> MQNWTLVWQDEFTNGISSDWVFETGNGNSGWGNNELQYYRRENATVENGNLVITAKRESIGGYNYTSTRMKTQGRKSWKYGKVEARIAMPSFMGSWPAFWMLGDNISSVGWPACGAIDIMEHVNTEAQTHGTIHWQDHNNTYANYSGSIP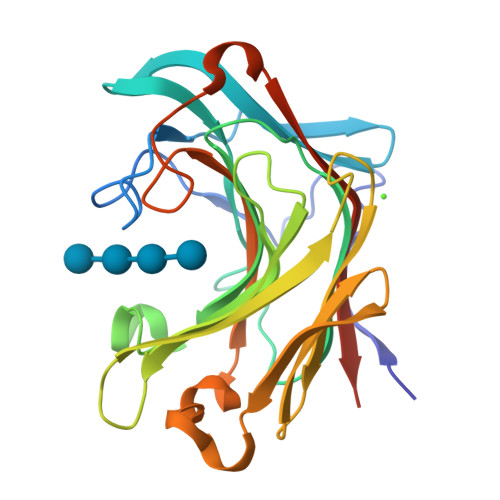VSSVTSYHIYTIEWDASVIKWFVDGNLYHEASIANGVNGTSEFHNNFFILLNMAIGGNWPGFNIDNNAFPARMLVDYVRVYQKTDLEHHHHHH>[3x]ETGDSITYNSGTSEFFDGDVFAIEVTADQSTDEIDIYLGASELSEKTDGEVNQDLSIEFTHQDSKLKYSTSTSDELRDIVTLTTYYEDGFDTEQDAIDAIKSDCYDLNQNGNGSGRYSRYYSVTSPVYDYEIYCFQKNEKLATPAYIDNPDEIFTAKAELQAGDKTIQSATLSNGDAGDGTVTDLGDSKISWNGNLDLGASEPENSRVIALYSNDFENGWRIGNKQSYEDYKTFIGGGDAYDLLIDWQDGTYTASEVEDELVNTDANQAVEEASSSTTDLVNAKVKDSSLDTGSFVYDTPELLSYPSF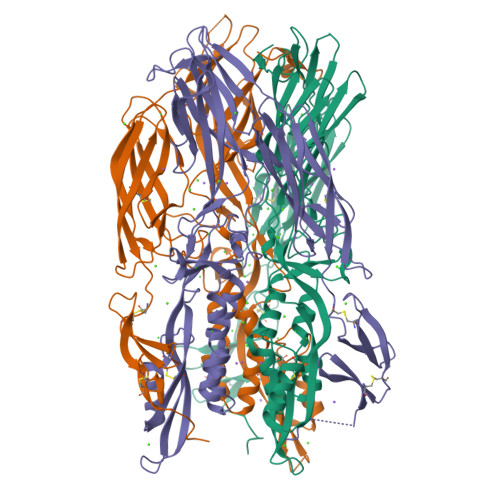TVYVDAGENGYIEVTKPTGDPDIISTSSTEIKEGDEGTVCATVENVGDGEGEFSGRLSSCGEGFSIVDDQNTKNVGAGESVTYSFDVAFSSVSSESKEISGSCTFEVNGVESSDSTSVSVTGIQQSECNPGDQRREKNENDRWEIYTCQDNGLTYEYDVTCAEDEKAVAQGDNQFSCEKQDDDSGGGDNTGSDSGLFSNLFGGSGSLEHHHHHHHH>MSLNGSRRIPQPIRWAMVGGGSQSQIGYIHRCAALRDNTFVLVAGAFDIDPIRGSAFGEQLGVDSERCYADYLSMFEQEARRAD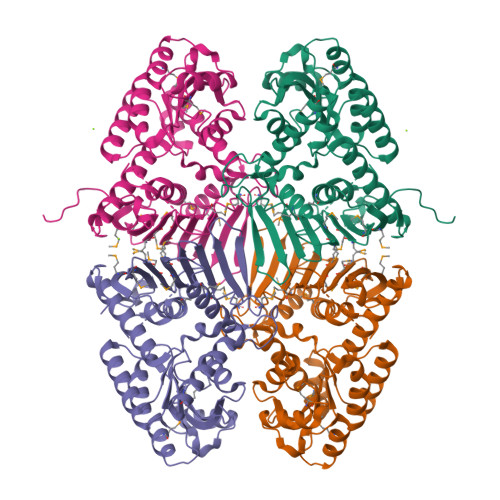GIQAVSIATPNGTHYSITKAALEAGLHVVCEKPLCFTVEQAENLRELSHKHNRIVGVTYGYAGHQLIEQAREMIAAGELGDVRMVHMQFAHGFHSAPVEAQSQATQWRVDPRQAGPSYVLGDVGTHPLYLSEVMLPDLKIKRLMCSRQSFVASRAPLEDNAYTLMEYEGGAMGMVWSSAVNAGSMHGQKIRVIGSRASLEWWDERPNQLSFEVQGQPAQILERGMGYLHPNALIDDRIGGGHPEGLFEAWANLYYRFALAMDATDRSDTQALSAVRYPGIDAGVEGVRWVERCVLSADNDSIWVAYEGHHHHHH[4x]> GHKSMENAAPSQDTDSPLSAASSSRNLEPHGKQPSLRAAKEHAMPKDLKKMLENKVIETLPGFQHVKLSVVKTILLKENFPYEGGLKIWECTFDLLAYFTKAKVKFAGKKVLDLGCGSGLLGITAFKGGSKEIHFQDYNSMVIDEVTLPNVVANSTLEDEENDVNEPDVKRCRKPKVTQLYKCRFFSGEWSEFCKLVLSSEKLFVKYDLILTSET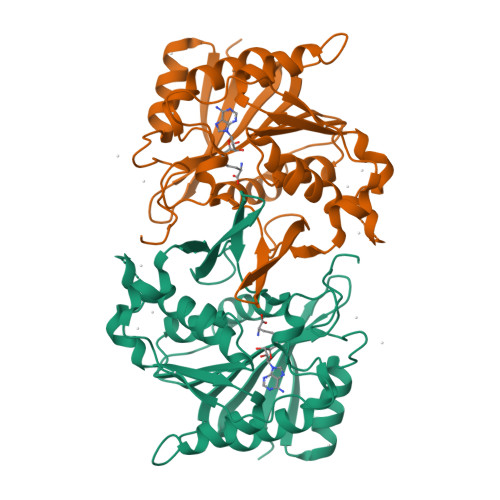IYNPDYYSNLHQTFLRLLSKNGRVLLASKAHYFGVGGGVHLFQKFVEERDVFKTRILKIIDEGLKRFIIEITFKFPG>GAMPPIFLPPPNYLFVRDVWKSNLYSEFAVIRQLVSQYNHVSISTEFVGTLARPIGTFRSKVDYHYQTMRANVDFLNPIQLGLSLSDANGNKPDNGPSTWQFNFEFDPKKEIMSTESLELLRKSGINFEKHENLGIDVFEFSQLLMDSGLMMDDSVTWITYHAAYDLGFLINILMNDSMPNNKEDFEWWVHQYMPNFYDLNLVYKIIQEFKNPQLQQSSQQQQQQQYSLTTLADELGLPRFSIFTTTGGQSLLMLLSFCQLSKLSMHKFPNGTDFAKY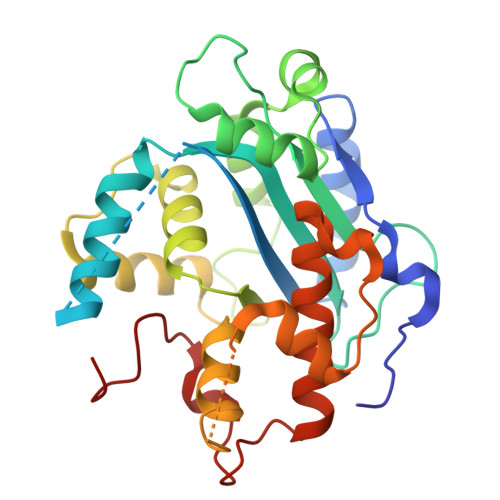QGVIYGIDGDQ[2x]>MPVFTASFQCVTLFGQPASAADAQPLLQGQRPFLHLHARRRRPCGPMLISKSPPYPASEETREWEADGQHEHTDELRETTTTMIDGIRTALRSIGEGEISISAYDTSLVALLKRLDGGDGPQFPSTIDWIVQNQLPDGSWGDASFFMMGDRIMSTLACVVALKSWNIHTDKCERGLLFIQENMWRLAHEEEDWMLVGFEIALPSLLDMAKDLDLDIPYDEPALKAIYAERERKLAKIPRDVLHSMPTTLLHSLEGMVDLDWEKLLKLRCLDGSFHCSPASTATAFQQTGDQKCFEYLDGIVKKFNGGVPCIYPLDVYERLWAVDRLTRLGISRHFTSEIEDCLDYIFRNWTPDGLAHTKNCPVKDIDDTAMGFRLLRLYGYQVDPCVLKKFEKDGKFFCLHGESNPSSVTPMYNTYRASQLKFPGDDGVLGRAEVFCRSFLQDRRGSNRMKDKWAIAKDIPGEVEYAMDYPWKASLPRIETRLYLDQYGGSGDVWIGKVLHRMTLFCNDLYLKAAKADFSNFQKECRVELNGLRRWYLRSNLEKFGGTDPQTTLMTSYFLASANIFEANRAAERLGWARVALLADAVSSHFRRIGGPKNSTSNLEELISLVPFDDAYSGSLREAWKQWLMAWTAKESSQESIEGDTAILLVRAIEIFGGRHVLTGQRPDLWEYSQLEQLTSSICCKLSRRVLAQENGESTEKV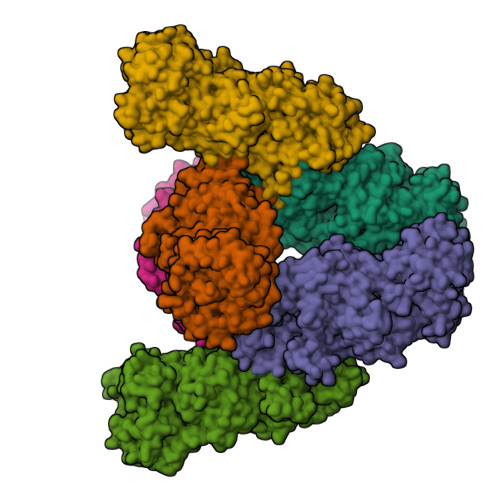EEIDQQVDLEMQELTRRVLQGCSAINRLTRETFLHVVKSFCYVAYCSPETIDSHIDKVIFQDVIEFHHHHHH[6x]Here, we have sought to generate high-resolution crystallographic structures of the cellular interacting fiber-knob domains of species D adenoviruses HAdV-D26 and HAdV-D48. The fiber-knob is the receptor interacting domain of the fiber protein, one of three major capsid proteins along with the hexon and penton base, as shown schematically in Fig. 1a. We next calculated the amino acid variability at each position in the aligned adenoviral fiber-knob sequences, which revealed regions of broad conservation corresponding to β-strands which make up the main fold of the fiber-knob trimer. Each monomer interacts with two neighbouring copies to form a homotrimer with 3-fold symmetry and a highly stable interface. Analysis of the adenovirus loops reveals an intricate network of polar interactions which stabilise their three-dimensional structures.

Most notably, vectors under development include those based on species D serotypes including HAdV-D26, which has entered Phase-III clinical trials as an Ebola vaccine and recently reported promising immunogenicity in an HIV trial. The HI loops of HAdV-D26K and HAdV-D48K are most homologous to those of HAdV-B35K and HAdV-D37K respectively in terms of amino acid sequence identity and spatial alignment. To investigate whether the different loop conformations were the product of flexibility, or restricted mobility we investigated the inter-loop interactions in the HAdV-D26K and HAdV-D48K structures. This analysis shows that the GH loop of HAdV-D26K (like those of HAdV-C5K, HAdV-D37K, and HAdV-D48K) does not extend directly away from the G and H β-sheets, but forms a β-hairpin that is maintained by seven polar contacts within the neighbouring IJ loop which restrict the loops’ orientation. The DG-loop of HAdV-D26K is calculated to have interaction energy of −6.5 kcal mol−1 in two separate stretches of this exceptionally long loop. Importantly, no strong contacts are found within the inter-monomer cleft. Loops which can occupy a CAR inhibitory conformation but have fewer stabilising contacts, such as that of HAdV-D26K, should be more permissive to CAR binding. HAdV-D26K shows a very low affinity interaction with CD46, however the kinetics are extremely fast making it impossible to measure an accurate KOn/Off at any of the concentrations measured, suggesting an unstable interface. The calculated KD for HAdV-D26K is seen to be more than 1.5 × 103 times lower than that of HAdV-B35K. We demonstrate that HAdV-D26 and HAdV-D48 fiber-knob domains have a weak ability to bind CAR, and negligible CD46 interaction, suggesting that these viruses are unlikely to utilise these proteins as a primary receptor in vivo.

> RRTLWTTPDTSPNCKMSTEKDSKLTLTLTKCGSQVLGNVSLLAVTGEYHQMTATTKKDVKISLLFDENGILLPSSSLSKDYWNYRSDDSIVSQKYNNAVPFMPNLTAYPKPSAQNAKNYSRTKIISNVYLGALTYQPVIITIAFNQETENGCAYSITFTFTWQKDYSAQQFDVTSFTFSYLTQE(2~{S})-2-[2-[4-(4-methoxyphenyl)phenyl]sulfanylphenyl]pentanedioic acid | C24 H22 O5 S | 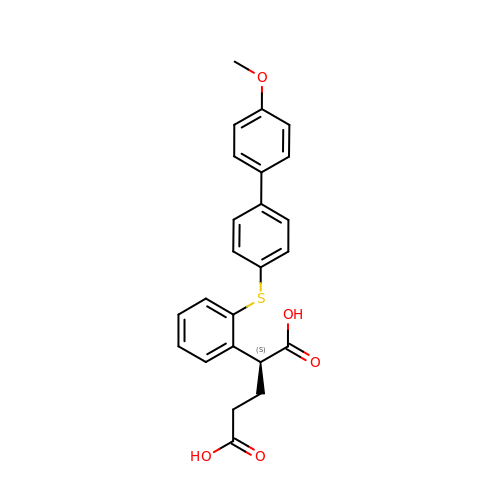KSEPBMMZVPGILK-NRFANRHFSA-N> MGTLEKKLDNLVNTILLKAENQHELLFGACQSDVK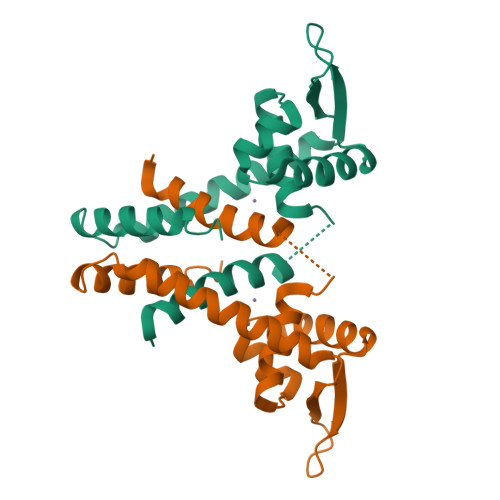LTNTQEHILMLLSQQRLTNTDLAKALNISQAAVTKAIKSLVKQDMLAGTKDTVDARVTYFELTELAKPIASEHTHHHDETLNVYNRLLQKFSAKELEIVDKFVTVFAEELEGLEHHHHHH>[2x]MGSSHHHHHHSSGLVPAGSMSQSPNTLANEETTSIDKSITMDMVSMNGEMFYKIANNDAMRPFFMTIVSDSNHWMFVSSNGGLTAGRKNAEYALFPYYTDDKITESADITGSKSIFQIQYNNELIVW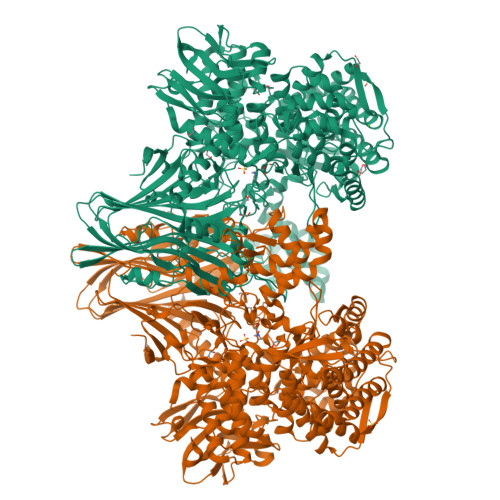EPFSERFTNKFKITRNLYKNYYGNKIIFEEINEDLGLTYRYQWCSSNQFGFVRKSELSNHSKNVYEISLLDGIQNIMPYGVSSDLQSSTSNLVDAYKRSELHPKSGLGIFALSAIIVDKAEPSEALKANIAWSLGLNNPKYLVSSLQLNHFRNGKSISPEDDIKGEKGAYFLNTVMTLEANTQKEWMIIANVNQDHSDIIAITETIQNNKKIAEDINTDIELGTKRLIELNASSDALQLTADNLRDTRHFSNTLFNIMRGGIFDNNYQIEKGDFSNYIKKANKLVFDKIDLNALGEIFSLNDLNEFASKQKDVDFDRLALEYLPLKFSRRHGDPSRPWNKFSINTQSEIDGSKVLDYEGNWRDIFQNWEALAHSFPNFIDSMIHKFLNASTFDGYNPYRVTKEGFDWETIEEDDPWSYIGYWGDHQIIYLLKFLEFIEKHQPGKLHSYFESECFVYAAVPYTIKPYEEILNNPKDTIGYNHEWEKVINERKKSIGADGALLKSNDKSIYHVNFIEKILATVLAKMSNFIPEAGIWLNTQRPEWNDANNALVGNGVSMVTLYYLRRFLKFFDQLLENSTLENIKISNEMVEFYHKVRETLMENQHLLAGSISDTDRKVILDKLGNAAADYRFQIYNSGFWGKKRTHSMQGLKNFTKVSLQFIDHSIKANQRPDKLYHAYNLMSVEKNKEIAISYLSEMLEGQVAVLSSGFLSSKENLAVLDGLKNSALFREDQYSYLLYPNKELPKFLDKNTISKEAVSKSELLSLLVSKSNKQVIEKDSIGEYHFNGEFNNASNLKQALEDLSQQNEYKDLVAKESKTVEAIFEDVFNHKAFTGRSGTFYGYEGLGSIYWHMVSKLQLAVLECCLKAVEEKESEEVIGRLLEHYYEINEGIGVHKSPSLYGAFPTDAYSHTPAGKGAQQPGMTGQVKEDILSRFGELGIFVKNGCLELNPCLLRKDEFLKEAKTFDYVTVNFQHQSLELVEKSLAFTYCQIPIIYKIANQKCIEVFTNDGKSAKAASLILDKQTSQDVFGRTGIINKIEVSILESDLR>SNADGLEGMDDPDATSKKVVPLGVEIYEINGPFFFGVADRLKGVLDVIEETPKVFILRMRRVPVIDATGMHALW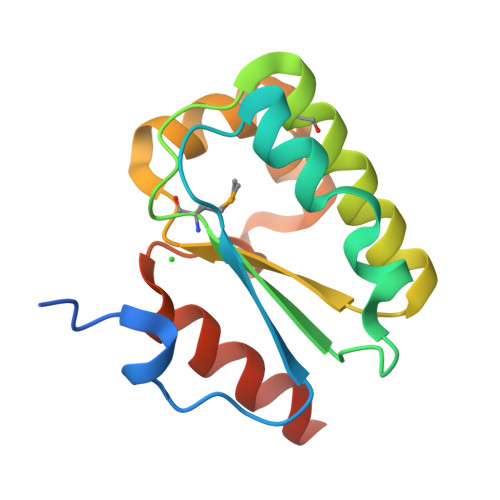EFQESCEKRGTILLLSGVSDRLYGALNRFGFIEALGEERVFDHIDKALAYAKLLVETAEER[2x]triptolide 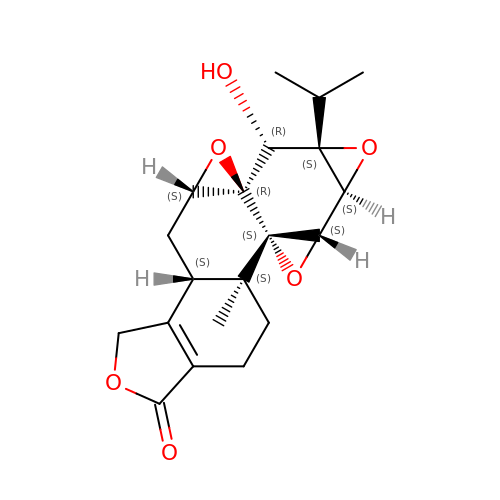| C20 H24 O6 | DFBIRQPKNDILPW-CIVMWXNOSA-N> LLDFDILTNDGTHRNMKLLIDLKNIFSRQLPKMPKEYIVKLVF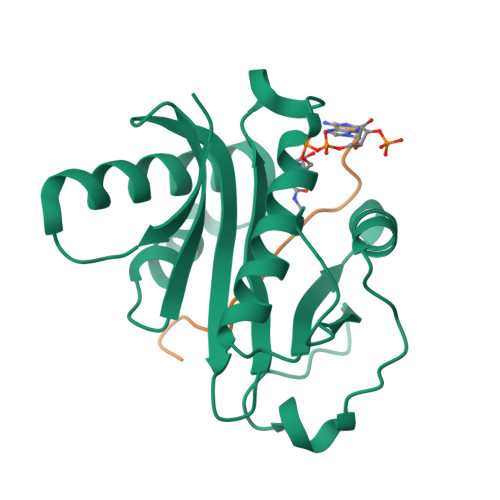DRHHESMVILKNKQKVIGGICFRQYKPQRFAEVAFLAVTANEQVRGYGTRLMNKFKDHMQKQNIEYLLTYADNFAIGYFKKQGFTKEHRMPQEKWKGYIKDYDGGTLMECYIHPYVDYGR;> QTARKSTGGKAPRKQLASK> MQASQFSAQVLDWYDKYGRKTLPWQIDKTPYKVWLSEVMLQQTQVATVIPYFERFMARFPTVTDLANAPLDEVLHLWTGLGYYARARNLHKAAQQVATLHGGKFPETFEEVAAL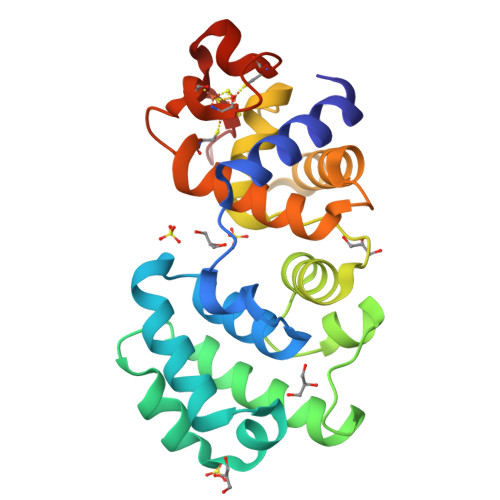PGVGRSTAGAILSLSLGKHFPILDGNVRRVLARCYAVSGWPGKKEVENKLWSLSEQVTPAVGVERFNQAMMDLGAMICTRSKPKCSLCPLQNGCIAAANNSWALYPGKKPK> MRRRAVLGGAVVYPEGPPPSYESVMQQQAAMIQPPLEAPFVPPRYLAPTEGRNSIRYSELSPLYDTTKLYLVDNKSADIASLNYQNDHSNFLTTVVQNNDFTPTEASTQTINFDERSRWGGQLKTIMHTNMPNVNEYMFSNKFKARVMVSRKAPEGVTVNDTYDHKEDILKYEWFEFILPEGNFSATMTIDLMNNAIIDNYLEIGRQNGVLESDIGVKFDTRNFRLGWDPETKLIM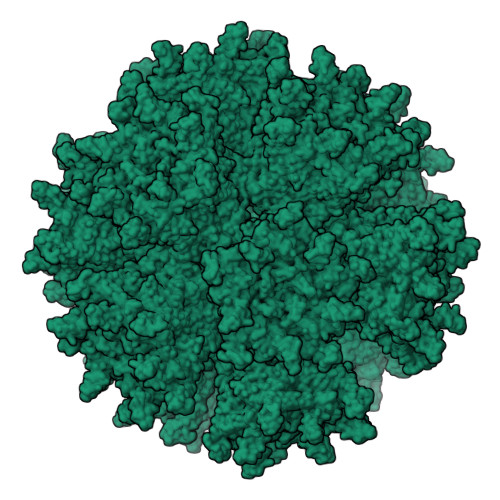PGVYTYEAFHPDIVLLPGCGVDFTESRLSNLLGIRKRHPFQEGFKIMYEDLEGGNIPALLDVTAYEESKKDTTTETTTKKELKIQPLEKDSKSRSYNVLEDKINTAYRSWYLSYNYGNPEKGIRSWTLLTTSDVTCGAEQVYWSLPDMMQDPVTFRSTRQVNNYPVVGAELMPVFSKSFYNEQAVYSQQLRQATSLTHVFNRFPENQILIRPPAPTITTVSENVPALTDHGTLPLRSSIRGVQRVTVTDARRRTCPYVYKALGIVAPRVLSSR>[3x]PTLEVYLPQGHSDERKASLIDGLTRATVDAIGAPAESVRILLTELPVSNIGL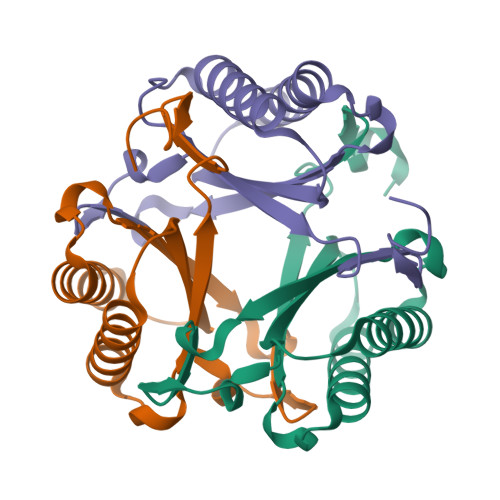GGKPTPAALPVIIAILIAGRTEAQKEALIAHLSETSASVLDVSLQSTRVMIKDIPNTDFGLGGKTARALGR The YfiBNR system contains three protein members and modulates intracellular c-di-GMP levels in response to signals received in the periplasm. YfiN is repressed by specific interaction between its periplasmic PAS domain and the periplasmic protein YfiR. YfiB is an OmpA/Pal-like outer-membrane lipoprotein that can activate YfiN by sequestering YfiR in an unknown manner. Previous studies suggested that in response to cell stress, YfiB in the outer membrane sequesters the periplasmic protein YfiR, releasing its inhibition of YfiN on the inner membrane and thus inducing the diguanylate cyclase activity of YfiN to allow c-di-GMP production.

We obtained two crystal forms of YfiB (residues 34–168, lacking the signal peptide from residues 1–26 and periplasmic residues 27–33), crystal forms I and II, belonging to space groups P21 and P41, respectively. The crystal structure of YfiB monomer consists of a five-stranded β-sheet (β1-2-5-3-4) flanked by five α-helices (α1–5) on one side. Each crystal form contains three different dimeric types of YfiB, two of which are present in both, suggesting that the rest of the dimeric types may result from crystal packing. Here, we refer to the two dimeric types as “head to head” and “back to back” according to the interacting mode, with the total buried surface areas being 316.8 Å2 and 554.3 Å2, respectively. The “head to head” dimer exhibits a clamp shape. The dimerization occurs mainly via hydrophobic interactions formed by A37 and I40 on the α1 helices, L50 on the β1 strands, and W55 on the β2 strands of both molecules, making a hydrophobic interacting core. The results showed that wild-type YfiB exists in both monomeric and dimeric states in solution, while YfiBL43P primarily adopts the monomer state in solution. The apo YfiB structure constructed beginning at residue 34 has a compact conformation of approximately 45 Å in length. Thus, YfiB alone represents an inactive form that may only partially insert into the PG matrix.

>GLSAEQIAVLQEQGFELRDEGWEFGMSSKVLFGNNLDRLNPDSRNTLTKIARALLAVDIDKVRLEGHTDNYGDEGYNQKLSERRAESVAAVFREAGMPAANIEVRGLGMSKPVADNKTRAGRSENRRVAIIVPAE[2x]>GGSGGSYRVVAYYISAGAYGRSYFPSDIDYSKVTHINYAFANIKDGEVVVGDPGVDDGGKNNFTALRKAKKAHPHLRNLISVGGWSWSSGFSDAAATPEARKRFADSAVAFIRKYGFDGVDIDWEYPVEGGAENMKHRPEDKQNYTLLTRSLREALDTAGKADGKYYELTTAVWGNDKFIANTEMDKVSRDFDFINVMSYDFNGTWNKFSGHNAPFVNDPAYDKPGIGKTFNVVSAVEAYLKAGVPADKLVVGVPLYGYSWKGCAAGERNGEYQDCNGKGRGTWEDGNLDFTDIEKNLLNKKGFKRYWNDTAKAAYLYNAETGEFVTYEDPQALKIKLDYIKSKGLGGAMYWEITADRK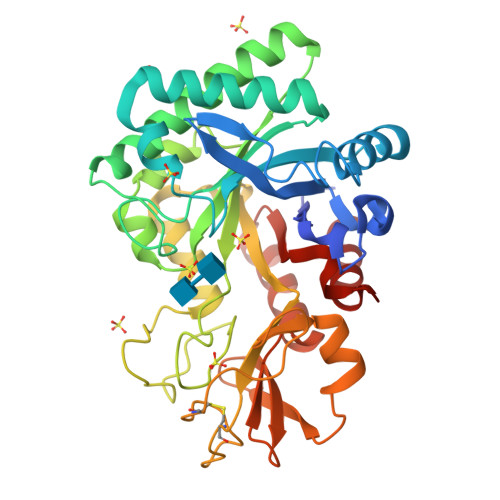QTLVNLIADELLT[2x]> MVAYPGPMPRSPSPGQTPDAPTSGGGSTDSTRQRIVAAAKEEFARHGIAGARVDRIAKQARTSKERVYAYFRSKEALYAHVAERETTALIEATQLDPADLPG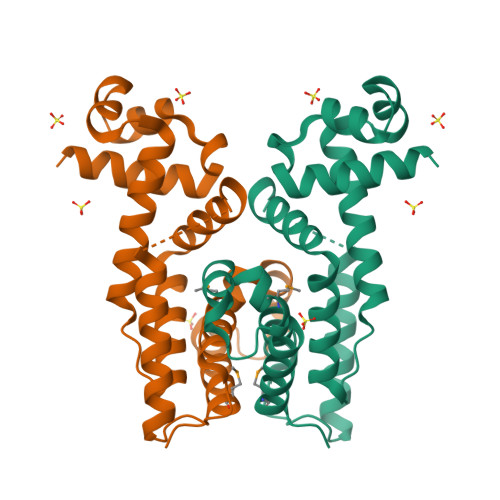YAGILFDHFAARPDHYRLITWGRLELAESADNTSGPLQATIAGKLDKLRDAQRIGLLDPAWDPVDVLALINQIAMTWAGQPEIAAAAADQAVDPSVTARRAALVTAVEHMFPRPDRDQRPNRLT> MSQEIRQNEKISYRIEGPFFIIHLMNPDNLNALEGEDYIYLGELLELADRNRDVYFTIIQSSGRFFSSGADFKGIAKAQGDDTNKYPSETSKWVSNFVARNVYVTDAFIKHSKVLICCLNGPAIGLSAALVALCDIVYSINDKVYLLYPFANLGLITEGGTTVSLPLKFGTNTTYECLMFNKPFKYDIMCENGFISKNFNMPSSNAEAFNAKVLEELREKVKGLYLPSCLGMKKLLKSNHIDAFNKANSVEVNESLKYWVDGEPLKRFRQLGSKQRKHRL;> ADVGSCSVGNNPLAQLHKHTQQNKSLQFNQKNNGRLNESPLQGTNKPGISEAFISNVNAISQENMANMQRFINGEPLIDDKRRMEIGPSSGRLPPFSNVHSLQTSANPTQIKGVNDISHWSQEFQGSNSIQNRNADTGNSEKAWQRGSTTASSRFQYPNTMMNNYAYASMNSLSGSRLQSPAFMNQQQSGRSKEGVNEQEQQPWTDQFEKLEKEVSENLDINDEIEKEENVSEVEQNKPETVEKEEGVYGDQYQSDFQEVWDSIHKDAEEVLPSELVNDDLNLGEDYLKYLGGRVNGNIEYAFQSNNEYFNNPNAYKIGCLLMENGAKLSEAALAFEAAVKEKPDHVDAWLRLGLVQTQNEKELNGISALEECLKLDPKNLEAMKTLAISYINEGYDMSAFTMLDKWAETKYPEIWSRIKQQDDKFQKEKGFTHIDMNAHITKQFLQLANNLSTIDPEIQLCLGLLFYTKDDFDKTIDCFESALRVNPNDELMWNRLGASLANSNRSEEAIQAYHRALQLKPSFVRARYNLAVSSMNIGCFKEAAGYLLSVLSMHEVNTNNKKGDVGSLLNTYNDTVIETLKRVFIAMNRDDLLQEVKPGMDLKRFKGEFSF

A prominent example is peroxisomal matrix proteins, most of which depend on the targeting factor Pex5 to localize and function correctly. One such example is the yeast Eci1 (Δ3, Δ2-enoyl-CoA isomerase 1), an enzyme that is essential for the β-oxidation of unsaturated fatty acids in peroxisomes. Although Eci1 contains a PTS1, its targeting to peroxisomes can occur independently of this signal. Using cryo-electron microscopy (cryo-EM), we resolved the structure of the Pex5–Eci1 complex, revealing a novel binding interface in addition to the PTS1-binding interface.

To gain molecular insight, we focused on the subset where Pex5 and the Eci1–Pex5 interface was most stable, containing only a single Eci1 subunit bound to Pex5. The maps from this subset were refined to 2.7 Å (1 Å=0.1 nm) globally, whereas Pex5 and the interface were resolved to 2.9 Å after local refinement of this region. Interestingly, there was electron density for an additional 21 residues at the Pex5 N-terminal region (276LVNDDLNLGEDYLKYLGGRVN296), which we name the Eci1-binding interface (EBI). This interface had not been observed previously in any other known Pex5 structures. Cryo-EM maps of the Pex5–Eci1 complex, containing the full-length Pex5, did not show electron density for the N-terminal domain (NTD) of Pex5 (up to residue E275). The first involves the C-terminal segment (268FRQLGSKQRKHRL280) of one out of the six Eci1 subunits, which includes the PTS1 (278HRL280) and interacted with the TPR3, TPR6 and TPR7 domains of Pex5. The PTS1-containing segment was located within a deep central cavity of the TPR domain and was reinforced by a network of hydrogen bonds formed between 278HRL280 and residues in TPR3, TPR6 and TPR7 of Pex5. Our structural analysis revealed a previously unidentified binding interface – the EBI, consisting of an elongated stretch of 21 mostly variable residues in the NTD of Pex5 (276LVNDDLNLGEDYLKYLGGRVN296). This stretch interacted with a distinct interface on Eci1, as well as with a few residues from the C-segment of Eci1 (F268, L271, and G272), suggesting that the EBI and the PTS1-binding regions work together to facilitate the interaction between Pex5 and Eci1.> ALNRKVKNNPDPTIYPVLDWNDIKFQDVIGEGNFGQVLKARIKKDGLRMDA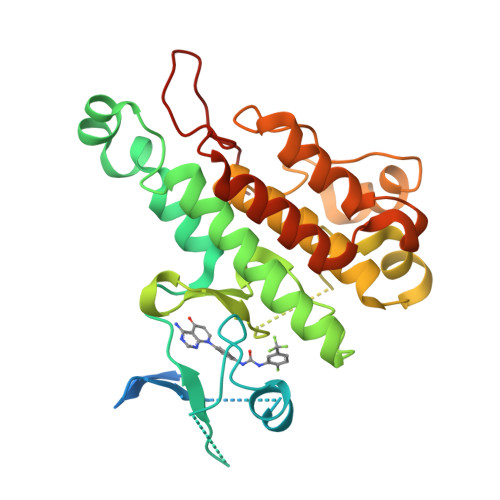AIKRMKEYASKDDHRDFAGELEVLCKLGHHPNIINLLGACEHRGYLYLAIEYAPHGNLLDFLRKSRVLETDPAFAIANSTASTLSSQQLLHFAADVARGMDYLSQKQFIHRNLAARNILVGENYVAKIADFGLSRGQEVYVKKTMGRLPVRWMAIESLNYSVYTTNSDVWSYGVLLWEIVSLGGTPYCGMTCAELYEKLPQGYRLEKPLNCDDEVYDLMRQCWREKPYERPSFAQILVSLNRMLEERKTYVNTTLYEKFTYAGIDCSAEE> LTPEQKQKKAALSASEGEEVPQDKAPSHVPFLLIGGGTAAFAAARSIRARDPGARVLIVSEDPELPYMRPPLSKELWFSDDPNVTKTLRFKQWNGKERSIYFQPPSFYVSAQDLPHIENGGVAVLTGKKVVQLDVRDNMVKLNDGSQITYEKCLIATGGTPRSLSAIDRAGAEVKSRTTLFRKIGDFRSLEKISREVKSITIIGGGFLGSEL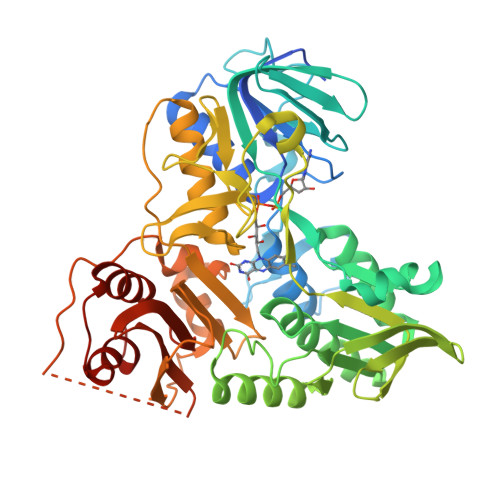ACALGRKARALGTEVIQLFPEKGNMGKILPEYLSNWTMEKVRREGVKVMPNAIVQSVGVSSGKLLIKLKDGRKVETDHIVAAVGLEPNVKLAKTGGLEIDSDFGGFRVNAELQARSNIWVAGDAACFYDIKLGRRRVEHHDHAVVSGRLAGENMTGAAKPYWHQSMFWSDLGPDVGYEAIGLVDSSLPTVGVFAKATAQDNPKSATEQSGTGIRSESETESEASEITIPPSTPAVPQAPVQGEDYGKGVIFYLRDKVVVGIVLWNIFNRMPIARKIIKDGEQHEDLNEVAKLFNIHED> SSLQGPELHGWRPPVDCVRANELCAAESNCSSRYRTLRQCLAGRDRNTMLANKECQAALEVLQE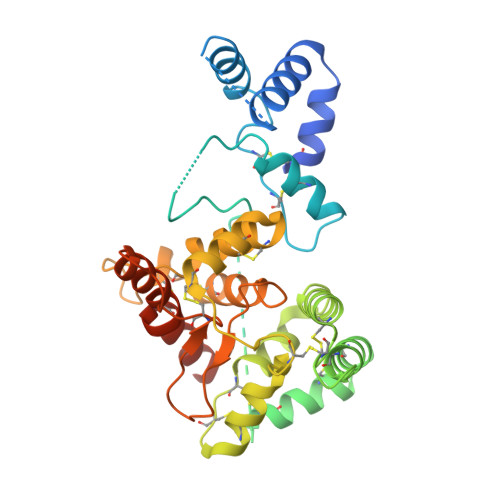SPLYDCRCKRGMKKELQCLQIYWSIHLGLTEGEEFYEASPYEPVTSRLSDIFRLASIFSGTGADPVVSAKSNHCLDAAKACNLNDNCKKLRSSYISICNREISPTERCNRRKCHKALRQFFDRVPSEYTYRMLFCSCQDQACAERRRQTILPSCSYEDKEKPNCLDLRGVCRTDHLCRSRLADFHANCRASYQTVTSCPADNYQACLGSYAGMIGFDMTPNYVDSSPTGIVVSPWCSCRGSGNMEEECEKFLRDFTENPCLRNAIQAFGNGTDVNGTHHHHHHHH> MSTPARRRLMRDFKRLQEDPPVGVSGAPSENNIMQWNAVIFGPEGTPFEDGTFKLVIEFSEEYPNKPPTVRFLSKMFHPNVYADGSICLDILQNRWSPTYDVS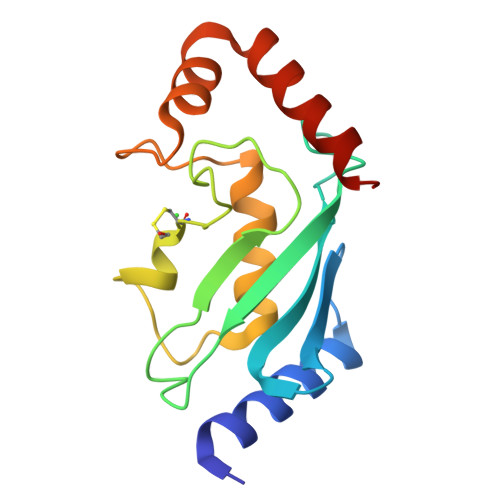SILTSIQSLLDEPNPNSPANSQAAQLYQENKREYEKRVSAIVEQSWNDS> MNDVEKLVKLLTSTDSETQKEAARDLAEIASGPASAIKAIVDAGGVEVLVKLLTSTDSEVQKEAARALANIASGPDEA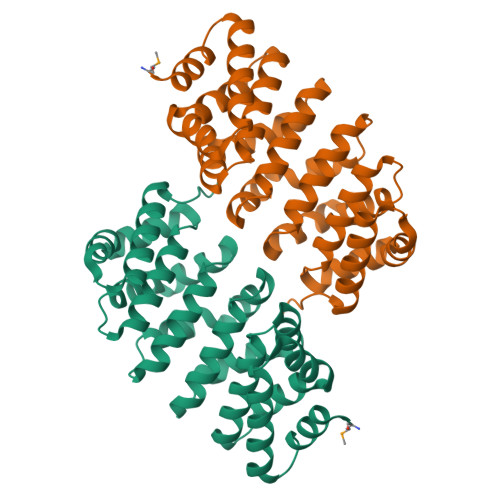IKAIVDAGGVEVLVKLLTSTDSEVQKEAARALANIASGPDEAIKAIVDAGGVEVLVKLLTSTDSEVQKEAARALANIASGPDEAIKAIVDAGGVEVLVKLLTSTDSEVQKEAARALANIASGPTSAIKAIVDAGGVEVLQKLLTSTDSEVQKEAQRALENIKSGGWLEHHHHHH>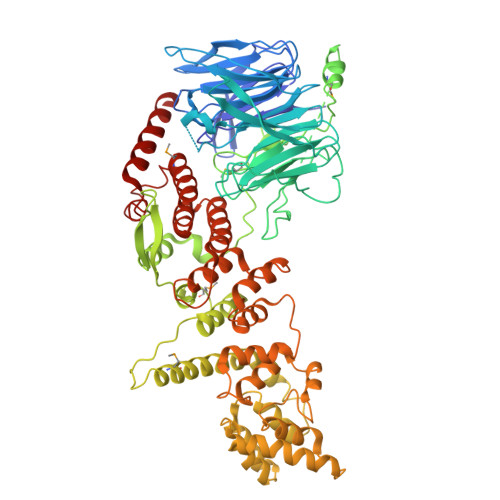 MVVIANAHNELIHDAVLDYYGKRLATCSSDKTIKIFEVEGETHKLIDTLTGHEGPVWRVDWAHPKFGTILASCSYDGKVLIWKEENGRWSQIAVHAVHSASVNSVQWAPHEYGPLLLVASSDGKVSVVEFKENGTTSPIIIDAHAIGVNSASWAPATIEEDGEHNGTKESRKFVTGGADNLVKIWKYNSDAQTYVLESTLEGHSDWVRDVAWSPTVLLRSYLASVSQDRTCIIWTQDNEQGPWKKTLLKEEKFPDVLWRASWSLSGNVLALSGGDNKVTLWKENLEGKWEPAGEVHQGGGGSGGGGATSKEFDGPCQNEIDLLFSECNDEIDNAKLIMKERRFTASYTFAKFSTGSMLLTKDIVGKSGVSIKRLPTELQRKFLFDDVYLDKEIEKVTIEARKSNPYPQISESSLLFKDALDYMEKTSSDYNLWKLSSILFDPVSYPYKTDNDQVKMALLKKERHCRLTSWIVSQIGPEIEEKIRNSSNEIEQIFLYLLLNDVVRASKLAIESKNGHLSVLISYLGSNDPRIRDLAELQLQKWSTGGCSIDKNISKIYKLLSGSPFEGLFSLKELESEFSWLCLLNLTLCYGQIDEYSLESLVQSHLDKFSLPYDDPIGVIFQLYAANENTEKLYKEVRQRTNALDVQFCWYLIQTLRFNGTRVFSKETSDEATFAFAAQLEFAQLHGHSLFVSCFLNDDKAAEDTIKRLVMREITLLRASTNDHILNRLKIPSQLIFNAQALKDRYEGNYLSE>MSLSDTIPVFDGHNDFLLRLLRNPANRETIWLKGDGTGHLDLPRMKEGGFAGGFFAIYVPSPQAHDAAHFEAMMDAPPFEL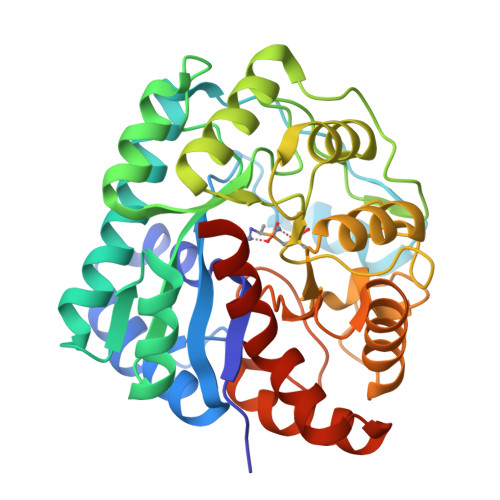PLPPMIRAEQAQPVALAMAGHLLWMERAARGRFKVCRTAAEVRSCHADGIVSGIMHMEGAEAIGADLDALHLFHSLGLRSLGPVWSRPTVFGHGVPFRFPGSPDTGEGLTEAGRRLVAECNRLKIMLDLSHLNEKGFDDVARLSDAPLVATHSNAHAVTPSTRNLTDRQLAMIRESRGMVGLNFATSFLREDGRRSAEMGWEPVLRHLDHLIDRLGEDHVGMGSDFDGATIPQGIADVTGLPALQAAMRAHGYDEPLMRKLCHENWYGLLERTWGEGHHHHHH[2x]> SLFEAWAKPVQPFAIWPGVWYVGTENLSSVLLTTPQGHILIDAGLDASAPQIRRNIEALGFRMADIRYIANSHARLDHAGGIARLKAWSGARVIASHANAEQMARGGKEDFALGDALPFPPVTVDMEAQDGQQWHLGGVTLAAIFTPGHLPGATSWKVTLADGKTLIYADSLATPGYPLINNRNYPTLVEDIRRSFARLEAQQVDIFLANHGERFGLMDKMARKARGENNAFIDKAGLARYVAQSRAAFEKQLAAQRAQP

Among the most effective bacterial resistance mechanisms are β-lactamases, a family of enzymes that are divided into four distinct classes. Classes A, C and D (serine-β-lactamases, SBLs) use a catalytic site serine residue to initiate inactivation of the antibiotic, while Class B (metallo-β-lactamases, MBLs) relies on a Zn2+-activated hydroxide. MBLs contain catalytic centres that can accommodate two closely spaced Zn2+ ions bound in the α and β sites with similar yet distinct sequence motifs (B1: His116, His118, His196 and Asp120, Cys221, His263 (i.e., HHH/DCH) for the α and β sites, respectively; B2: NHH/DCH; B3: HHH/DHH). For B3-type MBLs two variations of the canonical active site motif have been observed, QHH/DHH in GOB-1/18 from the opportunistic pathogen Elizabethkingia meningoseptica and HRH/DQK in SPR-1 from Serratia proteamaculans (variations shown in bold).

B3-RQK MBLs have three distinct aa variations in the active site motif, including two in the β site. We determined the crystal structures of the mature CSR-1 protein and CSR-1trunc, and compared them to structures of B3 and B3-Q MBLs. However, no metal ions were observed in the crystal structures of CSR-1 and CSR-1trunc, suggesting reduced metal ion affinity. To probe the role of these residues single, double and triple mutants of CSR-1trunc (i.e., CSR-1trunc,sm, CSR-1trunc,dm and CSR-1trunc,tm) were generated to create variants where either the α, the β or both metal binding sites are identical to the canonical B3 MBL motif. These mutations had no significant effect on the overall structures, however, in CSR-1trunc,sm electron density indicates the presence of one bound Zn2+ in the α-site, while in the double and triple mutants both the α- and β-sites are occupied by Zn2+ ions. The increasing Zn2+ binding capacity of CSR-1trunc as a function of introduced mutations was paralleled by enhanced ex vivo and in vitro activities, especially for the double and triple mutants; importantly, these two variants are also resistant to CA. Thus, the variations in the β-site of B3-RQK MBLs are responsible for the loss of catalytic activity and sensitivity to CA. When the weaker bound metal was removed (from the β site), a stable enzyme-inhibitor complex was only formed in CSR-1trunc and CSR-1trunc,sm, indicating that CA inhibits B3-RQK MBLs by displacing Zn2+ from the low affinity β site. Mutation of the B3-RQK active site to restore the native B3 motif resulted in increased metal affinity, catalytic activity and resistance to CA. This can be primarily attributed to the restoration of the canonical histidine in position 263 of the β-site, and raises the possibility of modifying CA to effectively bind in the presence of His263, thereby increasing the therapeutic range of this widely used antibiotic resistance drug.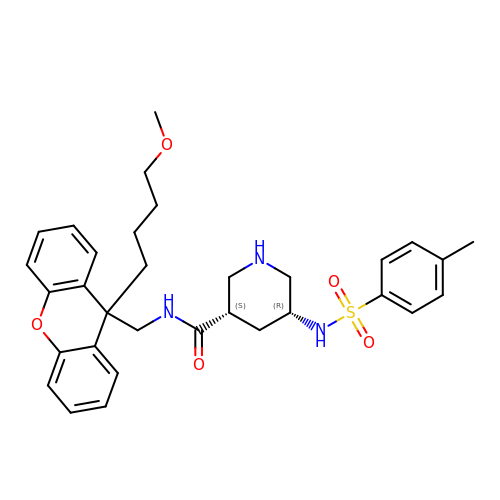(3S,5R)-N-{[9-(4-methoxybutyl)-9H-xanthen-9-yl]methyl}-5-{[(4-methylphenyl)sulfonyl]amino}piperidine-3-carboxamide | C32 H39 N3 O5 S | LBPUIWQYAGTBDC-LOSJGSFVSA-N>[4x]GSSYDWLNALNNLELLSLHSEILTQLRSRGVIRTKNNPVGDYAEWLVSNALGMTLLSNSSAGADAIDADGLKVQIKARRVTPDNPSRQLSALRNYEAADFDYLIAVIFDETYNILDAYKIPHEVIRDYARHSDHVNAHIVNLKGAILTDPRVSSIKEDLIVRSSASVNEAAMQT

The BisI family of restriction endonucleases is unique in requiring multiple methylated or hydroxymethylated cytosine residues within a short recognition sequence (GCNGC), and in cleaving directly within this sequence, rather than at a distance. We present the crystal structures of NhoI and Eco15I_Ntd (N-terminal catalytic domain of Eco15I) in the absence of DNA and in specific complexes with fully methylated GCNGC containing dsDNA. Both proteins are homodimeric, with each domain involved in target sequence recognition and catalysis. The crystal structures show that the modified cytosine bases are recognized in the context of double-stranded DNA, without base flipping.

NhoI is a typical BisI family member, Eco15I contains an additional domain at the C-terminus of the protein. We truncated the enzyme to the shortest active form of the catalytic domain (containing 173 amino acids) to increase the quality of crystals and refer to this truncated form as Eco15I_Ntd. Crystals grown in the absence of DNA contained either an NhoI dimer, or two Eco15I_Ntd dimers in the asymmetric unit. In the Eco15I_Ntd crystal structure without DNA, the relative orientation of the protomers is very similar to the orientation seen in the DNA complex. The region of β-stands β7 and β8 is disordered, so that DNA binding channel is open from the ‘top’, presumably to allow the enzyme to load onto DNA. However, the hairpin of β-stands β7 and β8 is much better ordered, likely because of crystal contacts to adjacent molecules. Together, the data suggest that NhoI and Eco15I_Ntd can latch onto DNA thanks to an opening of the DNA binding cleft, and due to flexibility of the β-hairpin that closes the DNA binding cleft at the top.> EVQIARKLQCIADQ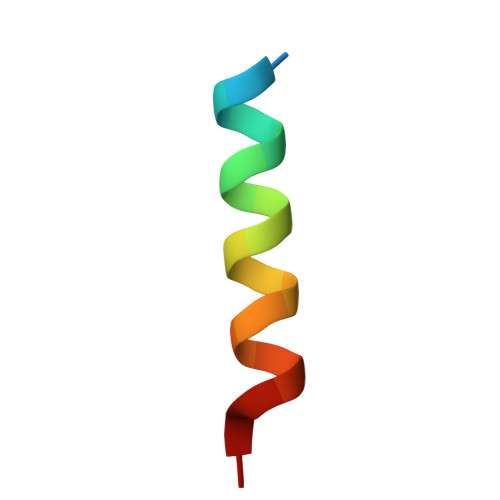FHRLHVQ2-[(PHENYLSULFONYL)AMINO]-5,6,7,8-TETRAHYDRONAPHTHALENE-1-CARBOXYLIC 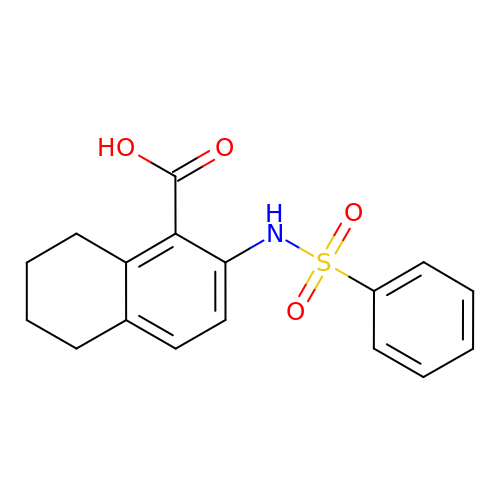ACID | C17 H17 N O4 S | RRXVUYHFDBLTEL-UHFFFAOYSA-N NaR belongs to the microbial rhodopsin family, whose members are widespread in the microbial world. In the dark state, all microbial rhodopsins contain all-trans retinal, which is bound to a specific Lys residue on the seventh helix (G helix) via a protonated Schiff base (PSB). During this photocycle, NaR achieves outward Na+ transport. After starting the photocycle, NaR captures Na+ from CP medium and then releases it to the extracellular (EC) medium.

We herein solved the structure of a NaR from the bacterium Indibacter alkaliphilus (hereafter, this NaR is abbreviated as IaNaR) and then found unique features in one protomer of the asymmetric dimer. The crystals were obtained by the lipidic cubic phase (LCP) at pH 5.1 (15). The crystals belonged to the P212121 space group, and the asymmetric unit contained two antiparallel protomers, which will be referred to as molecules A and B, respectively. The overall structures of the two protomers were similar to the reported KR2 structures, that is, they commonly contain a short N-terminal helix (N helix; residues 9–17) and consist of typical seven transmembrane domains. In molecule B, the three-residue cluster at the EC surface is disrupted, and in the vicinity of the PSB, the Arg108 sidechain lacks the interaction with Asp250 and is oriented toward the EC side. These differences from molecule A seem to be related to the large outward bending of the F' helix caused by unnatural interprotomer interactions. The EC end of this F' helix forms a hydrophobic interaction with the A helix (the first helix) from molecule B of the neighboring asymmetric unit. For IaNaR, the corresponding Asp115 is also oriented downward in both protomers, while the distances to the Schiff base nitrogen are somewhat longer (3.9 Å and 3.4 Å for molecules A and B, respectively). Thus, we assumed that molecule B mimics the Na+-releasing intermediate and then proposed a working hypothesis for the mechanism leading to the swing motion of the Arg sidechain.

>[2x]MENLGNATFENYIGLQDGFNEMAYQMVAHVLTLGYAVMLAGLFYFVLTIKTVAPRFRTSSVLSVVVMVSAFLLLYVQASNWTESFVFDTERGKYFLGEGNDLFNNGYRYLNWLIDVPMLLFQILFVVTLTKSNFSSIRNQFWISGTGMIVTGYIGQFYEVTDLTMFAIWGAISTVFFFHILWLMKKVIDEGKDGIPAKAQETLQSIWVLFLVSWMLYPGAYLMPHLAGIEGLFFSEIGVVARQITYTIADVSSKVIYGILLTNVAQVMSKEEGYLEHTTLEHHHHHH>MKLRGKILPLFVAIAMAIPAQAAEDRTIDLYAGQVRVIPTKPVKRVAIGDGKVLSTTVVDGNELLLLGDAEGETSLRVWFKDGSEAAYRVLVAPKNVGRAAEEMRELMGAEKSPAKIRVVGDHVVVDGKNLAPTTLARVRALQALYPKTIVLATPSPFDMEKMVWLDVNILEIRKSVLENFGVDWSKQIPGPFAAFGKDFVGPRNVATIPLGQDLTQPPVAGTGVRVTPPLGSLNGAIDLANLARPIAGTTNFGIITGVLSTINFALSNGDAYLIANPQLSARSGGRTDFLAGGQVPILQALAAGNAAFQNVTYKDYGIKLEFEPRVDDDNNVSMRVLADVSDIDPATSVSLNGFTVPGFITRRSNAEINVGDGQTMVISGLVNPKTAKNVSKLPWLGDIPILGNLFKSTNFQSGNTDLVILVTPRVVSAASLENIRQVS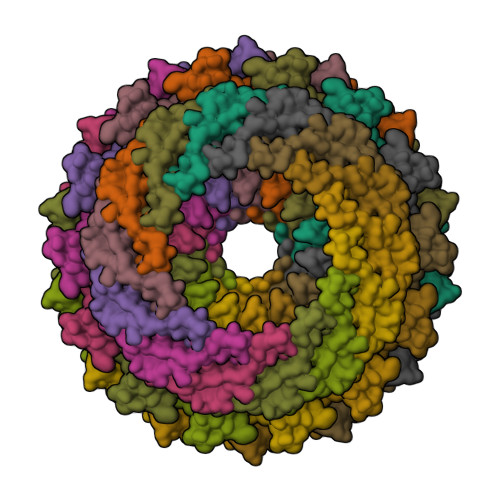QAVEMKDEYRNTLPKGSTTRDAVDRTLGSKTPYPETQAVPAPKPSLPLVVTQPPAAMPSDKE[14x]> MTVPVSVNYHFTRQCNYQCGFCFHTAKTSFVLPIEEAKKGLLMLMKAGMEKVNFSGGEPFLHDRGKFVGELVRYCKQELELPSVSIVSNGSLIRDNWFNKYGECLDILAISCDSFDEETNVLIGRRQKGKNHVEALRRVRDMCQQYKVAFKLNTVVNTYNKQEDMTSHIQELCPVRWKVFQCLVIAG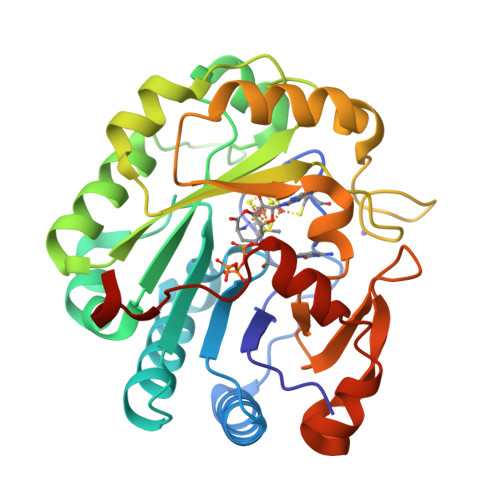ENSGEDALRDAEQFLVSNHEFDQFISRHASLECLVPESNEKMQNSYLILDEYMRFLDCTGGSKSPSKSILDVGVDQAMKFSGFDEKMFLKRGGKYVWSKADMKLDW> TSASEDIDFDDLSRRFEE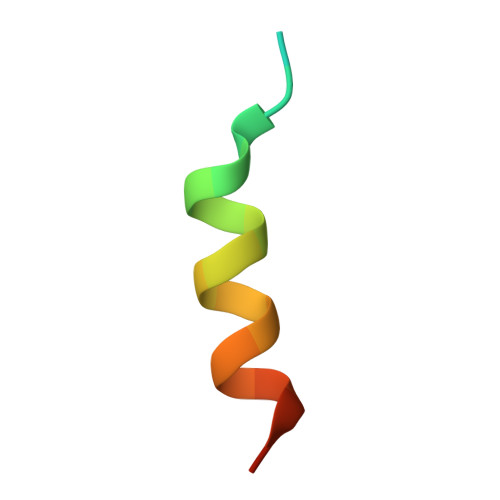LKKKT>[3x]RM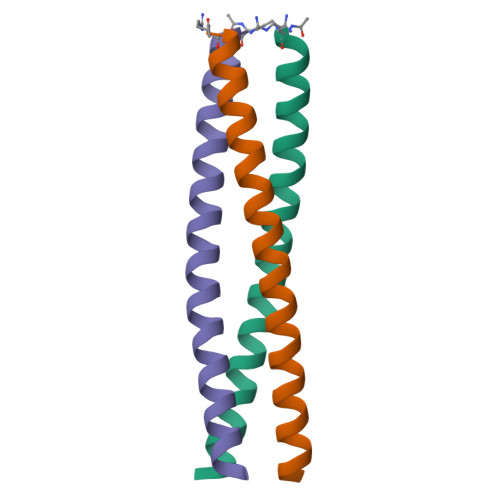KQIEDKIEEIESKQKKIENEIARIKKLLQLTVWGIKQLQARILX> MATQMQQRDNGEETLANIKHSARSELKDMNVSGLAGINIQAGGYDLTGLSLTDELIAQGLSNVGLLPFEHSRVVLELAEAITVTANNTDMGGSGQYCEQGAWRAWLHVGLNMAKHHVRIRSSAAMDFGTHRMMACDPASLDASTISAMSRNVTTATMNAVSREMKAMKALAAGRSRMSQSDIADNNDCRGFAFGVLSRMVMHNSARRHGVVNGRLQELGENDASTADTYLTWELACAHGKGEVAITPVPAAWLDPEAQLTGRERVFSEALARLVDPDVGCVHVKIDGVTQNAAENARVHYATRPDPMSWLDDNTGLSADSNAGRISGEHYTLWKGRHSKVHLTIQLKQLYHRMSTTAATAEPRADSIVYYLKGFEGLGACAEFLLANSRFGHHSFLPGVFGVTADVHEAAYAQNQALFLAGIGDRMPPATFTKAQLATATYALMRRYDISERTCHFAITTIGHMVAQTAVRDLNNGSLSPLPFRVNLSPFLVQGVQFWDMNDTEGSVSVHDMGIGKELLTATYALGAMASLAHVCEQGGTGEEMSAIEVSRFTDVHTVATDLFRKVVMTELGDLKLRGSEVTHSSQEALFAQKMKAVWSSMAEGSTRLYNLNQAYGPFVDVQLARIRSSFVRDIGASRQMMDASALIKHAQNVTYDWPQNESGCPVQFIALPVPSTITHYATPAIGTERWFATTRLNAAGSKVISEIRWTNGLNSDDRAGVHVFAYGRSTIVSSPLGCAEAMAAMVIAGEHKVVRRHTSIARAQSARTANIVAGAVLGARNGDMMTIIRPSTSVASSAVHLRGYIPMAAMNMLPITDGDCDLVVADTRTRPGRMSTSPEAHRRGVLASDYHVDIATDGNIRHVAREVYTVADIPTVSERVSGLALRPYERSCVRDASTLHSMLCGAVPLLYGGGEPMKLGDNTPVTNRQALRPPEYNRNPALRMPARFQMGTTACAFTKALGDVRAQMELREGDVVTEEVTEPDTTIVPQGSITERVVVGEMTEALIMADQPMFDQDVVQNIMYNSPGIRGTERANIQAELMAAKDWPSILQATAKS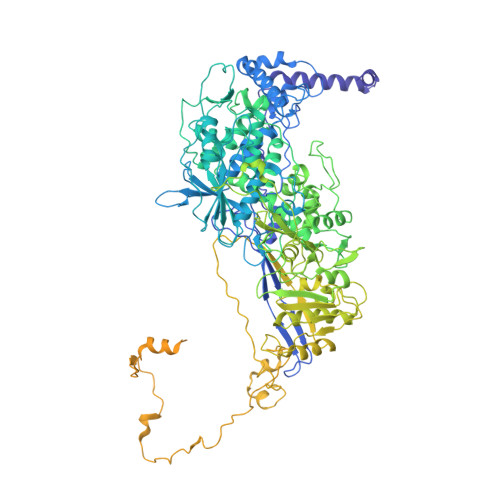SHGDIASAKTPYDLIKACKVDWSKVKGETQLKLIMNKIHPEYMTLSRAISAQVDARIVPNVPKSAMSTLLFWACATDMGLHTAVMANLAGLQRTTGFKGGIVYDLEGGANWPATDVRARIIEGWNAHARRIAQSGLISRDLTVMKIQHDMNADDIMALPAHIGDSWVLTIGELTANIATDEQSVAYAKDAQSAYYAIDRLRRLVAGREEGVDEILSKAEVMARVLAENKGLADDQALYHREWNRRTMAYVYMTTYLGSLDVEARLGVVSDDAYAERRAEWKAERAKLAVPAVSGQGQGRR> MREKPKYLPPTLRDKNRYIAFQVIGERPFKKDEIKKAVWEASLSALGYLGSARA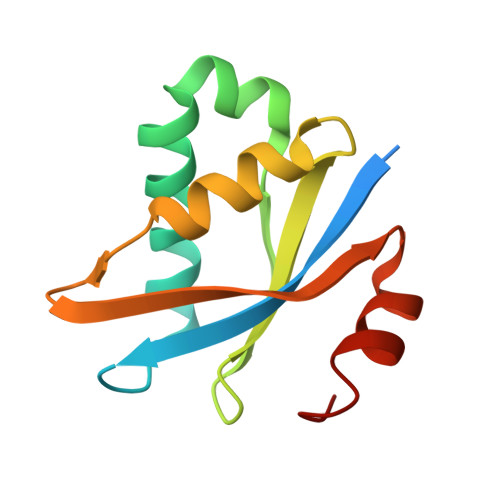KPWFIKFDEKSQTGIVRVDRKHVEELRFALTMLTEINGSKVIFRTLGVSGTIKRLKRKFLAEYGWR>DLSQCDREPIHLLGGIQSHGVLLAFRGPDRLLEVVSANAQALLGRPPETLLGQPVGRVLPAEVLAQWEPLVARGSVRVVLPAGAYRALLHESDGLTVLELEPAELQPGMEETALEVVRRLVSPLAGVKGTQALLQTAADTVRALTGFDRVMVYRFDADWHGEVLAESKRGGMDGFLGMHFPATDIPVQARALYTRNPLRLIADARARPVPLLPPVVPALGRPLDLSNSALRSVSPVHLEYLRNMGVGASFSLSLLKEGVLWGLIACTHLEPLHISHERRRACEVLTQLLALQLSAEERAAEASEDAHRAALLGQLATAMGEGGTLEEVLEKESERVLALTGAAG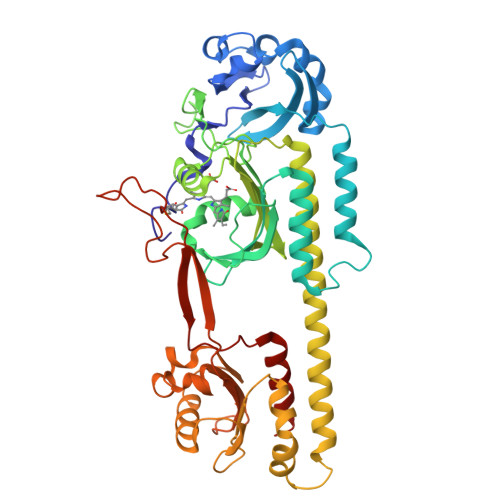VALLLGEEPLLVGCTPAQDEVEALVAWLATQPFQTSFHTDRLGTVYPPLAARADVAAGILAVRLAPAAARFAIWFRPEVARTISWAGNPRKPAEPEPGHQRLHPRGSFQAWEETVRDTSLPWKRADLGAAEGFRGAL[2x]> MSNWVMQEENKQGNLTPLFEELLQQCPPGGQNKTAHMVSAYQLAQGNWMPTSCHVFMGTISARRTKTHPYEAYVKLRELVEEHKMKTLCPGSSLGKHNDWIIGKIKYQGNLRTKHMLNPGKVAEQLCREGHRHNVYNKTIGSVMTATGIRLEKLPVVRAQTDTTNFHQAIRDKIDKEENLQTPGLHKKLMEVFNALKRPELESSYDAVEWEELERGINRKGAAGFFERKNIGEILDSE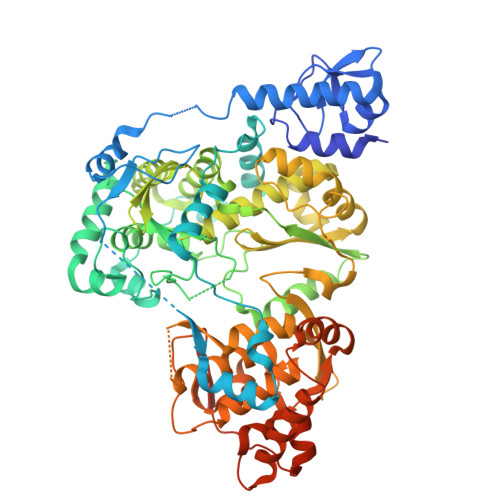KNKVEEIIDNLKKGRNIKYYETAIPKNEKRDVNDDWTAGDFVDEKKPRVIQYPEAKTRLAITKVMYKWVKQKPVVIPGYEGKTPLFQIFDKVKKEWDQFQNPVAVSFDTKAWDTQVTTKDLELIKDIQKYYFKKKWHKFIDTLTMHMTEVPVICADGEVYIRKGQRGSGQPDTSAGNSMLNVLTMVYAFCEATGVPYKSFDRVAKIHVCGDDGFLITERALGEKFASKGVQILAEAGKPQKITEGDKMKVAYQFDDIEFCSHTPIQVRWSDNTSSYMPGRNTTTILAKMATRLDSSGERGTIAYEKAVAFSFLLMYSWNPLIRRICLLVLSTELQVKPGKSTTYYYEGDPISAYKEVIGHNLFDLKRTSFEKLAKLNLSMSVLGAWTRHTSKRLLQDCVNMGVKEGNWLVNADRLVSSKTGNRYIPGEGHTLQGRHYEELVLARKQINNFQGADRYNGSSSHHHHHH1-(5-cyanopyrazin-2-yl)-3-(5-phenyl-1H-pyrazol-3-yl)urea 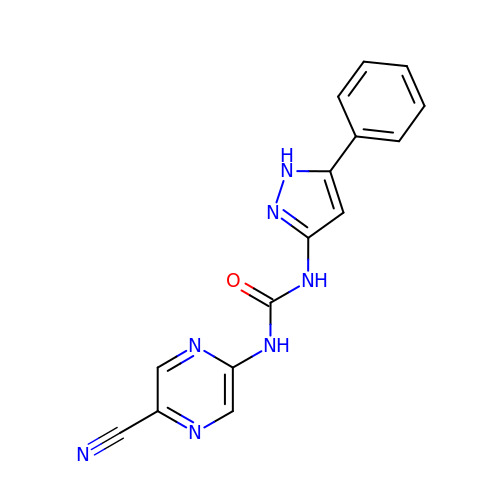| C15 H11 N7 O | CUGADHZZTWSNMF-UHFFFAOYSA-N>[4x]VGYGDITQVETSGASS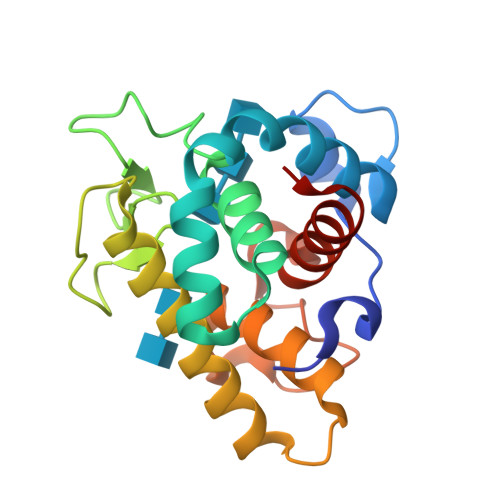KTSRQDKLEYDGVRASHTMAQTDAGRMEKYKSFINNVAKKHVVDPAVIAAIISRESRAGNVIFNTTPPGWGDNYNGFGLMQVDKRYHEPRGAWNSEEHIDQATGILVNFIQLIQKKFPSWSTEQQLKGAIAAYNTGDGRVESYESVDSRTTGKDYSNDVVARAQWYKKNGF> DKKAYFYHSSFQILNVEYTEALNSPATHEYRTLSE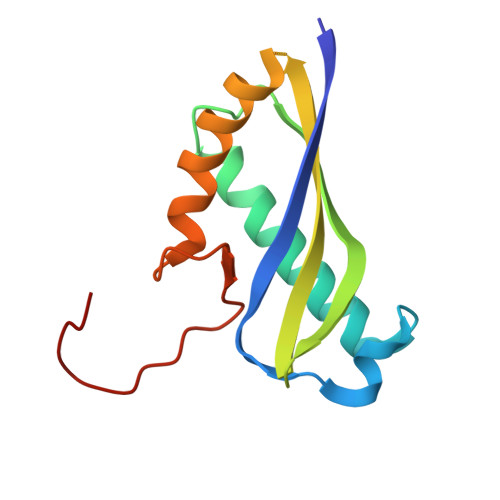RIEAMITDEFRGSSLKSEFIRTHVVKLRKEGTGVVADVVMKFRSSKRNNRKVMKTRIQSVLRRLSSSGNLEIAPSNEITSLTDQDT>[6x]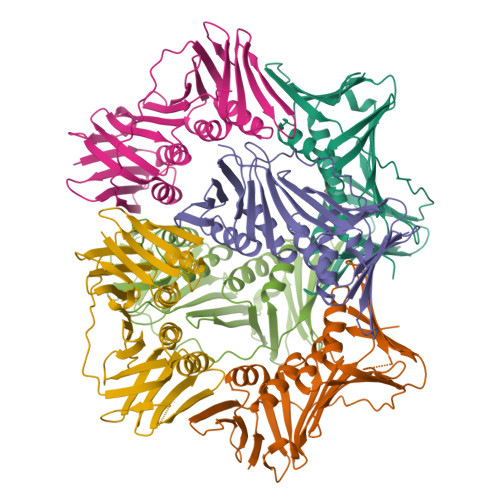MLEAQVQFASLWKRLVECINGLVNEANFDCNPGGLSVQAMDSSHVALVHMLLRDDCFVKYQCGRNSILGLNLASLSKVLKIVDSNDSLSLRHDDDSDVVTLTSENPEKTRKCEYQLKLLEIEAESMGIPEMDYRSTVTLNSAEFAKIVRDMQVFGDTVTIAISKEGVKFSSSGDVGQGYTFLQAAGVSDRSTKSEVKAEVKAEARDDDEEPLSRKYGKADSSANAIGVEVTMEEPITLSFALRFMGIFAKGSTLSERVTLKFAKDSPCMVEYGIDNVGYLRYYLAPKVDDAE Despite their differences, both complexes have integrated the large Tra1 (Transcription-Associated protein 1) subunit, an essential and highly conserved 433 KDa protein that belongs to the Phosphoinositide 3-Kinase-related kinase (PIKK) family of cellular regulators, which includes mTOR, DNA-PKcs, ATM/Tel1, ATR/Mec1 and SMG-1 (Baretić and Williams, 2014; Lempiäinen et al., 2009). PIKKs are protein kinases that have diverse regulatory functions in transcriptional regulation, DNA repair, cell growth, metabolic control and mRNA surveillance but Tra1 is the only member that is catalytically inactive, due to loss of the DFG motif within the kinase active site. Although lacking catalytic activity, Tra1 is critical for coactivator function as it is a direct target for multiple activators and enables the activities of SAGA and NuA4 to be directed at specific genes in order to stimulate their expression. Tra1 has the domain structure characteristic of PIKK family proteins, consisting of HEAT, FAT, FRB, Kinase and FATC domains arranged sequentially from N- to C- terminus (Baretić and Williams, 2014; Lempiäinen et al., 2009).

We over-expressed and purified S. cerevisiae Tra1 from its native host and determined its structure by single-particle cryo-EM to a resolution of 3.7 Å. Sidechains were visible throughout the reconstruction and an atomic model was built entirely de novo with 3474 residues (93%) assigned with excellent stereochemistry, representing the first atomic structure for this member of the PIKK family. Using that analogy, Tra1 can be broadly separated into four topological regions which we have termed Finger, Ring, Clasp and Head. The Finger, Ring and Clasp regions lie within the HEAT domain, whereas the Head region contains the FAT, FRB, Kinase and FATC domains. However, although the relative positions of the catalytic, activation and phosphate-binding loops of mTOR/DNA-PKcs are preserved in Tra1, the critical residues required for ATP/Mg binding and catalysis are not conserved, and the Tra1 activation loop contains an 18-residue insertion compared to its counterparts in the catalytic PIKKs. The relative juxtaposition of FRB and kinase domains also differ as the DNA-PKcs and mTOR FRB domains are positioned away from the active site cleft, whereas the Tra1 FRB domain occludes it, contacting the LBE (mLST8-Binding-Element) on the opposite site of the cleft. The FATC domain is integral to the kinase domain and is sandwiched between the LBE and the Kinase C-terminal lobe, forming a plug over a large hydrophobic cavity within the kinase domain. The interface is localized to one side of of Tra1, primarily around the FAT domain at TPR repeats T1-T7 (residues 2572–2830) but also at the C-terminal half of the Ring at repeats H41-H44 (residues 2150–2350), which clearly represent sites of intermolecular contact between Tra1 and the remaining SAGA subunits.

> MDYKDHDGDYKDHDIDYKDDDDKMSLTEQIEQFASRFRDDDATLQSRYSTLSELYDIMELLNSPEDYHFFLQAVIPLLLNQLKEVPISYDAHSPEQKLRNSMLDIFNRCLMNQTFQPYAMEVLEFLLSVLPKENEENGILCMKVLTTLFKSFKSILQDKLDSFIRIIIQIYKNTPNLINQTFYEAGKAEQGDLDSPKEPQADELLDEFSKNDEEKDFPSKQSSTEPRFENSTSSNGLRSSMFSFKILSECPITMVTLYSSYKQLTSTSLPEFTPLIMNLLNIQIKQQQEAREQAESRGEHFTSISTEIINRPAYCDFILAQIKATSFLAYVFIRGYAPEFLQDYVNFVPDLIIRLLQDCPSELSSARKELLHATRHILSTNYKKLFLPKLDYLFDERILIGNGFTMHETLRPLAYSTVADFIHNIRSELQLSEIEKTIKIYTGYLLDESLALTVQIMSAKLLLNLVERILKLGKENPQEAPRAKKLLMIIIDSYMNRFKTLNRQYDTIMKYYGRYETHKKEKAEKLKNSIQDNDKESEEFMRKVLEPSDDDHLMPQPKKEDINDSPDVEMTESDKVVKNDVEMFDIKNYAPILLLPTPTNDPIKDAFYLYRTLMSFLKTIIHDLKVFNPPPNEYTVANPKLWASVSRVFSYEEVIVFKDLFHECIIGLKFFKDHNEKLSPETTKKHFDISMPSLPVSATKDARELMDYLAFMFMQMDNATFNEIIEQELPFVYERMLEDSGLLHVAQSFLTSEITSPNFAGILLRFLKGKLKDLGNVDFNTSNVLIRLFKLSFMSVNLFPNINEVVLLPHLNDLILNSLKYSTTAEEPLVYFYLIRTLFRSIGGGRFENLYRSIKPILQVLLQSLNQMILTARLPHERELYVELCITVPVRLSVLAPYLPFLMKPLVFALQQYPDLVSQGLRTLELCIDNLTAEYFDPIIEPVIDDVSKALFNLLQPQPFNHAISHNVVRILGKLGGRNRQFLKPPTDLTEKTELDIDAIADFKINGMPEDVPLSVTPGIQSALNILQSYKSDIHYRKSAYKYLTCVLLLMTKSSAEFPTNYTELLKTAVNSIKLERIGIEKNFDLEPTVNKRDYSNQENLFLRLLESVFYATSIKELKDDAMDLLNNLLDHFCLLQVNTTLLNKRNYNGTFNIDLKNPNFMLDSSLILDAIPFALSYYIPEVREVGVLAYKRIYEKSCLIYGEELALSHSFIPELAKQFIHLCYDETYYNKRGGVLGIKVLIDNVKSSSVFLKKYQYNLANGLLFVLKDTQSEAPSAITDSAEKLLIDLLSITFADVKEEDLGNKVLENTLTDIVCELSNANPKVRNACQKSLHTISNLTGIPIVKLMDHSKQFLLSPIFAKPLRALPFTMQIGNVDAITFCLSLPNTFLTFNEELFRLLQESIVLADAEDESLSTNIQKTTEYSTSEQLVQLRIACIKLLAIALKNEEFATAQQGNIRIRILAVFFKTMLKTSPEIINTTYEALKGSLAENSKLPKELLQNGLKPLLMNLSDHQKLTVPGLDALSKLLELLIAYFKVEIGRKLLDHLTAWCRVEVLDTLFGQDLAEQMPTKIIVSIINIFHLLPPQADMFLNDLLLKVMLLERKLRLQLDSPFRTPLARYLNRFHNPVTEYFKKNMTLRQLVLFMCNIVQRPEAKELAEDFEKELDNFYDFYISNIPKNQVRVVSFFTNMVDLFNTMVITNGDEWLKKKGNMILKLKDMLNLTLKTIKENSFYIDHLQLNQSIAKFQALYLRFTELSERDQNPLLLDFIDFSFSNGIKASYSLKKFIFHNIIASSNKEKQNNFINDATLFVLSDKCLDARIFVLKNVINSTLIYEVATSGSLKSYLVEDKKPKWLELLHNKIWKNSNAILAYDVLDHHDLFRFELLQLSAIFIKADPEIIAEIKKDIIKFCWNFIKLEDTLIKQSAYLVTSYFISKFDFPIKVVTQVFVALLRSSHVEARYLVKQSLDVLTPVLHERMNAAGTPDTWINWVKRVMVENSSSQNNILYQFLISHPDLFFNSRDLFISNIIHHMNKITFMSNSNSDSHTLAIDLASLILYWENKTLEITNVNNTKTDSDGDVVMSDSKSDINPVEADTTAIIVDANNNSPISLHLREACTAFLIRYVCASNHRAIETELGLRAINILSELISDKHWTNVNVKLVYFEKFLIFQDLDSENILYYCMNALDVLYVFFKNKTKEWIMENLPTIQNLLEKCIKSDHHDVQEALQKVLQVIMKAIKAQGVSVIIEEESPGKTFIQMLTSVITQDLQETSSVTAGVTLAWVLFMNFPDNIVPLLTPLMKTFSKLCKDHLSISQPKDAMALEEARITTKLLEKVLYILSLKVSLLGDSRRPFLSTVALLIDHSMDQNFLRKIVNMSRSWIFNTEIFPTVKEKAAILTKMLAFEIRGEPSLSKLFYEIVLKLFDQEHFNNTEITVRMEQPFLVGTRVEDIGIRKRFMTILDNSLERDIKERLYYVIRDQNWEFIADYPWLNQALQLLYGSFNREKELSLKNIYCLSPPSILQEYLPENAEMVTEVNDLELSNFVKGHIASMQGLCRIISSDFIDSLIEIFYQDPKAIHRAWVTLFPQVYKSIPKNEKYGFVRSIITLLSKPYHTRQISSRTNVINMLLDSISKIESLELPPHLVKYLAISYNAWYQSINILESIQSNTSIDNTKIIEANEDALLELYVNLQEEDMFYGLWRRRAKYTETNIGLSYEQIGLWDKAQQLYEVAQVKARSGALPYSQSEYALWEDNWIQCAEKLQHWDVLTELAKHEGFTDLLLECGWRVADWNSDRDALEQSVKSVMDVPTPRRQMFKTFLALQNFAESRKGDQEVRKLCDEGIQLSLIKWVSLPIRYTPAHKWLLHGFQQYMEFLEATQIYANLHTTTVQNLDSKAQEIKRILQAWRDRLPNTWDDVNMWNDLVTWRQHAFQVINNAYLPLIPALQQSNSNSNINTHAYRGYHEIAWVINRFAHVARKHNMPDVCISQLARIYTLPNIEIQEAFLKLREQAKCHYQNMNELTTGLDVISNTNLVYFGTVQKAEFFTLKGMFLSKLRAYEEANQAFATAVQIDLNLAKAWAQWGFFNDRRLSEEPNNISFASNAISCYLQAAGLYKNSKIRELLCRILWLISIDDASGMLTNAFDSFRGEIPVWYWITFIPQLLTSLSHKEANMVRHILIRIAKSYPQALHFQLRTTKEDFAVIQRQTMAVMGDKPDTNDRNGRRQPWEYLQELNNILKTAYPLLALSLESLVAQINDRFKSTTDEDLFRLINVLLIDGTLNYNRLPFPRKNPKLPENTEKNLVKFSTTLLAPYIRPKFNADFIDNKPDYETYIKRLRYWRRRLENKLDRASKKENLEVLCPHLSNFHHQKFEDIEIPGQYLLNKDNNVHFIKIARFLPTVDFVRGTHSSYRRLMIRGHDGSVHSFAVQYPAVRHSRREERMFQLYRLFNKSLSKNVETRRRSIQFNLPIAIPLSPQVRIMNDSVSFTTLHEIHNEFCKKKGFDPDDIQDFMADKLNAAHDDALPAPDMTILKVEIFNSIQTMFVPSNVLKDHFTSLFTQFEDFWLFRKQFASQYSSFVFMSYMMMINNRTPHKIHVDKTSGNVFTLEMLPSRFPYERVKPLLKNHDLSLPPDSPIFHNNEPVPFRLTPNIQSLIGDSALEGIFAVNLFTISRALIEPDNELNTYLALFIRDEIISWFSNLHRPIIENPQLREMVQTNVDLIIRKVAQLGHLNSTPTVTTQFILDCIGSAVSPRNLARTDVNFMPWF> GSQNQERLCAFKDPYQQDLGIGESRISHENGTILC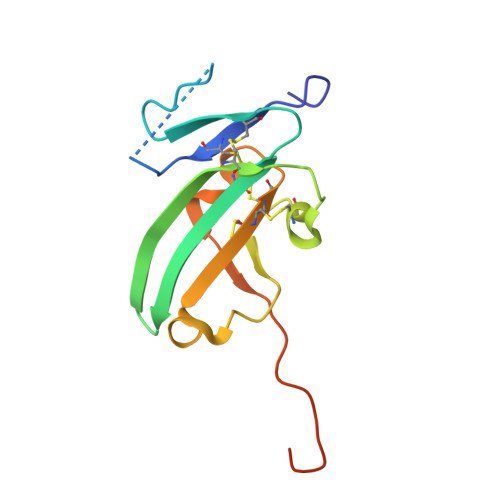SKGSTCYGLWEKSKGDINLVKQGCWSHIGDPQECHYEECVVTTTPPSIQNGTYRFCCCSTDLCNVNFTENFPPPDTTPLSPPHSFNRDET αHBs are oligomers of 5 or more α-helical peptides that assemble into coiled-coil structures with central solvent-accessible channels. We targeted two properties of αHBs: oligomeric state, which directly affects the internal diameter of the channel; and the identities of channel-facing residues, which fine tune this dimension and introduce different chemistries. The αHBs are loaded with an environment sensitive dye (in this case, 1,6-diphenyl-1,3,5-hexatriene, DPH) that binds within the channels and fluoresces. Accordingly, challenging the array with analytes leads to differential displacement of the dye across the array to give a fluorescent fingerprint.

Despite the requirements for aliphatic residues at a and d, up to 40% of these can be changed to other side chains without compromising barrel integrity. We introduced mutations at one or two of these sites to generate four groups of αHB: Group I had entirely hydrophobic interiors, but with different sizes and shapes of channel; Groups II and III had polar uncharged or polar charged residues, respectively, at specific points along the channel; and Group IV had aromatic residues installed in their channels. Finally, seven Group IV designs incorporated single Tyr at a or d sites, or Trp residues at a sites. Finally, one third of the designs were crystallized and yielded 12 X-ray crystal structures, all of which were open αHBs with fully accessible channels. Conversely, the FAs generate signal through interactions with the more-hydrophobic and aromatic-containing channels (Group I and IV).

>[2x]XGEIAQAYKEIAKALKEIAWALKEIAQALKGX> SNKVGTLQAQVEATQKQKAQPIDANRKYDYKLQYYLNDYVYAYFTLPQEGDKQQAQVEHLNSFYNFVPDVKAQGQVRNPSTLLDSQLVTVEGKVATYKVKYKEMIQHDKDTEEKELVTGFNIPFDEKEGKYYVSGLPWFSAIESSQAGYFSEDDQLQLTANDHVSDSQHKKVEKFLKVFFTNYTTNQDNLNLIAKNVAIVANTTFKTIDYTYLKKDRADLIAYVQATFEVGGTTHSENFTFTLSEKDKSYYVTKLEHTIPLNYANDKD

The main model of our study is OrfG, the sole VirB8-like protein of the conjugative and integrative element ICESt3 found in the Gram-positive bacterium Streptococcus thermophilus. Bioinformatic analysis using constrained consensus TOPology prediction (CCTOP) predicted that OrfG consists of a single transmembrane α helix (residues 37 to 57) followed by a large soluble domain (OrfG64–331). This soluble region comprises two NTF2-like domains OrfG64–204 and OrfG223–331 (referred to hereafter as D1 and D2, respectively). Our data confirm that VirB8-like proteins are predominantly extracellular components, assembling into a conserved pattern, which serves as a building block of the DNA translocation channel.

We determined the crystallographic structure of OrfGExt at a resolution of 1.83 Å. As anticipated, it exhibits two NTF2-like domains D1 and D2, connected by a long-extended linker. In domain D1, the region between residues 92 and 204 forms two successive α helices followed by a long loop (instead of a third α helix typically observed in VirB8 and VirB8-like proteins) and then a highly curved antiparallel β sheet composed of four strands wrapped around the first α helix. The domain D2 (residues 228 to 321) adopts a similar fold to domain D1 [root mean square deviation (RMSD) = 2.57 Å for 78 aligned residues] but with a shorter α helix 2 and shorter loops between the strands and once again lacks a third α helix before entering the β sheet. A notable feature common to these two domains is the high proportion of aromatic residues in their core, predominantly phenylalanines and tyrosines (D1: four Phe + four Tyr; D2: seven Phe + two Tyr), at the interface between the helix 1 and the β sheet. In the crystal, OrfGExt forms a complex consisting of three intertwined protomers related by a threefold axis. The six NTF2-like domains are arranged in an almost flat triangle, with three domains D1 in the center and three domains D2 at the vertices. The notable feature of this arrangement is that each domain D1 not only faces the others (distance from center to center: 30 Å) but interacts with the domain D2 of the neighboring monomer (at 24 Å) instead of its own one positioned far away (52 Å), thanks to the long linker that stretches to wrap around the domain D1 of that neighbor. The D1 domains show minimal interaction (273 Å2 in OrfG, 444 Å2 in TcpC) and do not significantly contribute to the trimer stability, while the D1:D2′ interface represents a sufficient contribution to maintain the assembly (910 Å2 in OrfG, 965 Å2 in TcpC). In the crystal structure of OrfG, the trimers display no discernible interactions between them that could suggest a higher-order assembly.> MKMTSIQQRAELHRQIWQIANDVRGSVDGWDFKQYVLGALFYRFISENFSSYIEAGDDSICYAKLDDSVITDDIKDDAIKTKGYFIYPSQLFCNVAAKANTNDRLNADLNSIFVAIESSAYGYPSEADIKGLFADFDTTSNRLGNTVKDKNARLAAVLKGVEGLKLGDFNEHQIDLFGDAYEFLISNYAANAGKSGGEFFTPQHVSKLIAQLAMHGQT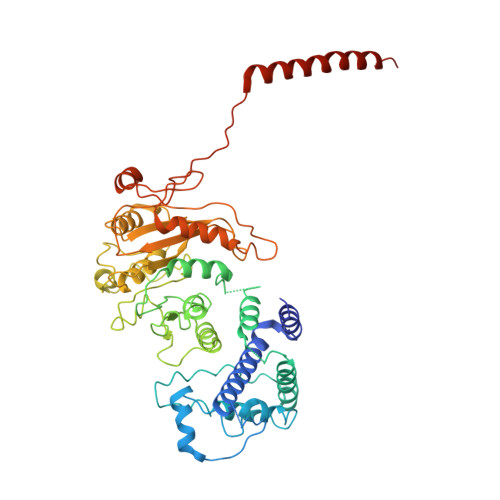HVNKIYDPAAGSGSLLLQAKKQFDNHIIEEGFFGQEINHTTYNLARMNMFLHNINYDKFDIKLGNTLTEPHFRDEKPFDAIVSNPPYSVKWIGSDDPTLINDERFAPAGVLAPKSKADFAFVLHALNYLSAKGRAAIVCFPGIFYRGGAEQKIRQYLVDNNYVETVISLAPNLFFGTTIAVNILVLSKHKTDTNVQFIDASELFKKETNNNILTDAHIEQIMQVFASKEDVAHLAKSVAFETVVANDYNLSVSSYVEAKDNREIIDIAELNAELKTTVSKIDQLRKDIDAIVAEIEGCEVQK> KPHISALNAPQLDQRYKNEFTIGAAVEPYQLQNEKDVQMLKRHFNSIVAENVMKPISIQPEEGKFNFEQADRIVKFAKANGMDIRFHTLVWHSQVPQWFFLDKEGKPMVNETDPVKREQNKQLLLKRLETHIKTIVERYKDDIKYWDVVNQVVGDDGKLRNSPWYQIAGIDYIKVAFQAARKYGGDNIKLYMNDYNTEVEPKRTALYNLVKQLKEEGVPIDGIGHQSHIQIGWPSEAEIEKTINMFAALGLDNQITELDVSMYGWPPRAYPTYDAIPKQKFLDQAARYDRLFKLYEKLSDKISNVTFWGIADNHTWLDSRADVYYDANGNVVVDPNAPYAKVEKGKGKDAPFVFGPDYK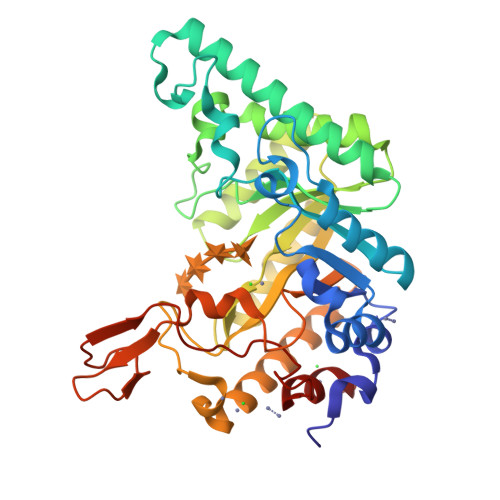VKPAYWAIIDHK>MLRLKTQDSRLKTQDSRLKTQDSRLKTQDSFSVDDNGSGNVFVCGDLVNSKENKVQFNGNNNKLIIEDDVECRWLTVIFRGDNNYVRIHKNSKIKGDIVATKGSKVIIGRRTTIGAGFEVVTDKCNVTIGHDCMIARDVILRASDGHPIFDIHSKKRI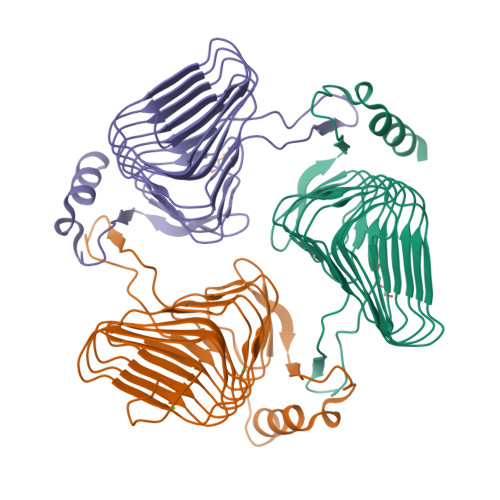NWAKDIIISSYVWVGRNVSIMKGVSVGSGSVIGYGSIVTKDVPSMCAAAGNPAKIIKRNIIWARTDKAELISDDKRCSSYHAKLTQLEHHHHHH[3x]>[4x]GPLGSLSTKRLRVLELYSGIGGMHYALNLANIPADIVCAIDINPQANEIYNLNHGKLAKHMDISTLTAKDFDAFDCKLWTMSPSCQPFTRIGNRKDILDPRSQAFLNILNVLPHVNNLPEYILIENVQGFEESKAAEECRKVLRNCGYNLIEGILSPNQFNIPNSRSRWYGLARLNFKGEWSIDDVFQFSEVAQKEGEVKRIRDYLEIERDWSSYMVLESVLNKWGHQFDIVKPDSSSCCCFTRGYTHLVQGAGSILQMSDHENTHEQFERNRMALQLRYFTAREVARLMGFPESLEWSKSNVTEKCMYRLLGNSINVKVVSYLISLLLEPLNF

For example, C5-methylation of C38 in the tRNA anticodon-loop by the methyltransferase Dnmt2 was shown to protect tRNAs from cleavage, which in turn has an impact on Dicer-2-dependent siRNA pathways. Recently, the C38 methylation of tRNAAsp in S. pombe was found to depend on the presence of queuosine (Q), a hypermodified nucleoside at position 34 of tRNAAsp, tRNAAsn, tRNATyr, and tRNAHis10. Here we demonstrate that Q34 of tRNAAsp solely is sufficient to increase Dnmt2 catalytic efficiency. We present the crystal structure of S. pombe Dnmt2 and propose a model of the Dnmt2-tRNA complex, based on in silico docking and mass spectrometric analysis of cross-links obtained from the Dnmt2-tRNA complex, showing that Q34 is part of the active site.

For further insights into the activation of Dnmt2 by Q we solved the spDnmt2 crystal structure in complex with S-adenosyl-homocysteine (SAH) at 1.7 Å resolution by molecular replacement. This structure comprises all amino acids from position 5 to the C-terminal end, including loop regions, and exhibits an overall simiIar fold with the Dnmt2 crystal structures from human (hsDnmt2)16 and the pathogenic amoebae E. histolytica (ehDnmt2)17. In the spDnmt2 structure we were able to build a loop of 20 amino acids starting with Cys80, which was proved to be important for catalysis in hsDnmt2 and therefore is referred to this loop as the “active site loop”. This loop is presumably unstructured in solution as the electron density for the corresponding amino acids was only observed for one of the four Dnmt2 molecules in the asymmetric unit, and this loop adopted a defined conformation due to formation of crystal contacts with another Dnmt2 molecule in the crystal lattice. Interestingly Pro83 in this loop exhibits a cis-peptide conformation in chains A and B of the crystal structure. Analysis of spDnmt2 electrostatic surface potentials unveils predominantly positively charged surface around the SAH indicating possible interaction with the tRNA phosphate backbone. However, the structure exposes a strongly negatively charged cavity in close proximity to the sulfur of SAH formed by the catalytic residue Glu121, which is also conserved in hsDnmt2 and ehDnmt2. This cavity might accommodate the base of cytosine C38, which needs to be flipped out in order to be methylated. The resulting model of the tRNA Dnmt2 complex has the tRNA placed with the anticodon stem in a positively charged groove around the active site. The modeled Dnmt2-tRNA complex reveals Q34 positioned close to the active site but simultaneously too distant from the catalytic residues to directly participate in the methyltransfer reaction.> HRFRVCALGAAFCVARRWRSGGGPGDRRVRTDWYRCYPSLMEEKDRDMYHCYYPYLFDHGDKMSLYPKIPDNPREWQVEQLQTTYDAIREDKYDAFVRLRAKFPELYQDTYAWDNPPPFGEFNMFYSVRFGMIGVKAFTCKDYDDLGNQFDCTAFWFPDNQIVKHSTRNGDVGTDKVYVGAMNVPVEFHKPHVAAFYKAAGVPVKHVSAGFPVTPDAYAPVGTKLDVRHFKPGQEVTITFQNTDYGYQGVMFRHGFDGGYVWLGDSKWQRRPGCMGAEGQKRIYPGHRMAGQTGASAETYDGVPVWRIDYKNSLIYLPTLIDADVGTYVKFRDTINTKGYTLWNEHRGTPPFPTFIPSEEEDLSKLATDEGQLTSPPLYMYFRDEFAAAQLVTQADVEDAKSAKPATAAPKKKVYDLKKYTEARKKYRKNLQKARKYKLMGVRTRAHEKQQEARRAKILKYKRVKT;> MLRLTQAVLRVQSHQKKRAQHPNAGTRFGRVYNRGFVRYGFGGFGMSVYSSKKDRTFKVMPVPPPPPATTAVEQRDDFADNRGLSATTRTLSPTFRMFALEDGGVLVSHPSHAQIMRWNQRVHTEEGKAANSTVMDEYVNSRIQAIIADNTIENTSLSQWRKAHMWNVIKSHGKLQRRWGTPDFVMGARSTLYNN;> MSRNGELCLQRIIVSYSPNKGNPAMRQFMATHLPEFHRQYPQVKIDIRPRQWPESSITGIYRDGSEKAYSIRFLSSMGINVRFHRLVNEGNDYNHSFSASHLHLQRRSVQGTWNPYLWNYEGTRARHKPPAQWSRKLTEKEWDYYVQQYGAQMKAEEDTIADRVRRYTDIPEASTEEVNQRWKEHVMPRLQTDLEYNLSHWKKQHRTGAGRPAPPTLNEYSLFSVPDHSSLGQDAIDMLRRREAQREEDWWRERKGQLKPPE;> MRYCRPSRPLVLARASSVLSSSRTFHSQHRTPIIPQVHVHDEPTAQRIHVGYYLHRHPVVKHSPHPLETEMGYLLEREQQRYSRHESAESATAFFASRGQTIDILGRTDPNQIKGNFFGLELYQDAMKVVMQRYTPEKRLTSADLWQPNALGDAPPPRHTLHRKLDDFLYLIVQEGATGKWTIPHTARKDDESLRMTADRAISSQNSEGLDCYVWSNAPQATVFLKDDNTRLFIYAATYLAGRPQFASFEPKPKDHAWVTRHELLQYSDTFKSAELLKALLDISADGTFEA;> MQPRRMAGHFNPTPQANSLAATHYAHTPELRHMADGAAMSLSGQRIPLLKPTLSKWSRQLRSDIYDELLKLPLRYALHDFRTLQAHIHAVPATATNASCTAAAGERLPPGVYHASSGLSSASPDAPAYYAVAGRDSAVGYAPPLGPADPVDVIPFFVHRSSNGHLPGKVYSMNAKTLMPAFYMRIQNIEGDMFRFEEELMKIFPTKKIFVRSHSVYVYNVNLDGRAVLHHWLLGLGF;> MTAPASHYTFANLKKLGLCAPQVALSRQPRLRPHVGHLNGLVYPLPYYAMWRGNHDKYTYNQATPARWGEGNTNTMYHQHYAHAKCPTDYGRGGREFQFLSVKRGKLKRKPLPTVQYVDPNSKPQWVFKSWHNPLSAPSMWEREVQYPEHTPAHTGAKRPLAVVAPKTSHKHLFLMHMEKVTVTVSPLLFGYGHTLQKAALDFYRRGLSARSPFPSDKMFLYYSIDHITPKIEVTWLDGSVYVPPLIEGVKAQDLIQMVMEQAWLAADRMSAEGRVLNPIAIDDYKWEQLIAFKQKRAKGAEAAKGGAKKK;> MLRRSPVPRRYRTAWRELLHPLPVWARRQQWLKRDTVEMNEAILREPYYRIKTFAQPAAFVSPRVSESAAHEPDTQQSSRYGVDRQLRGPRRAVSPERLQELREQLQFVGSIGPKVPPAAGAGTAYQDEYGTRLRPRYPQSWDTVPPHQPSRSEI;> MAFRGSSARLAATPGVGIAPETTPVKYVPEMLNIQNAKWWNGRGKPVYRSTYNEKSWLEKARWGAFTKGSRPVMRQRYSAAALKEALEMVPEGFETCDVPRPPQRIRAQSEGVVGRWYTNYWTLHSVRYQCQLAGVEWQFGERQRPRTNYDEPHMYTDFEETKAIRDYRSRWINVNRSLVGMSRRMKESEEEARYLHFKKVQDTFWSNRKVLVNRIKSMHNQGTLQSAKDLPIKTINIKAFLAE;> MHLHISSIPHRNSNNSKGGVLDATGPMLSAKRGALLLQAYHRPGEVISYKAGDYHLVPKKFTVGKRIAVRSYLDRNRTELSDRTFMPQKNWFRPYDLQDGCFDRDHERLSYRFYNLETKVIWKAFDTPELIGMLLHDETVKGNSGMYAPDMLDAALHYTREARYWRCIGITKPFYDRNTLRAHCWEDNGLQVGTLVMSQAMRHALMDLERAVRRKELGLEPNYLWDRWGPIGFIDGARADYLPRFEHNPYVDPDGVDVTEIDVLPFNTHEQIRERYRDFIEPDTAPFEEVFRSPSHGSLTTLADIPNASVVALYKDLKLKAGTPVAGDAVELAPADVRTLFYLSANPEWRAVADGKASWEEVVDAMQPVQAELDEKIDAARLLQNTRHNAERVRAFFEEKCGFHDFMYTPDKTITAAVLCYLTELRRICTETAWGAALAKCLTDMERVQGMGRDAFLVYRHIEDAILDKKRRLWAGRFAGESHEESTLDYLLENFGRRAERPRNVGTTGVEFDREQEPIGRQVQRRVLDSDKANKLAEIRRSRGKMWSKKRSVFDALHEKQLQNFNYGVH;> MPAYSEVKGTCGTPVLDQLIGYYVNIQSRKMYYKDFLRIEHQAVRWAFADIRKNSEALAHGLLQTGVRPGDRVLAIQPCNCETFVLQLSCAKIGALLCIVPQDTISADKLRFYLNEFQPRHLVAREWINVPEMKQGELVERNMHFWDTIYNVIPELGLSYPGQKFQWVHSQEFYYLKKIIITDHNMNLLGVTPMRKMLVWGPFSYYEQRLRRLSALLHPDDPVLALEDPNPAMEDKLHITYSHRNCVNAGFLFGQLMQLKAETRFGVMPNHHTDPIGAIIAPYAALTSGAVLVHIHSDMFTDDHAINGIEKLCVEEVETLVGRKADFDLILKHAGNFDADQFEHLRSVVIFEDGIEAPVSEEYLNKLSKALSLDDVYVFRGPIEASYMLTWRTLKKGSQGMVPHVEAKVVGDRGTSDAKVLVAGTRGNLRLKGPHVTAGYYNNAGLMTELIDEHGFASTSREAMIDGKDNITLMSAQTY;> MCTRVFDVSQRFILLVSLPPLSLSLRPSCCSRKAATRRRRSTASVLLATDALSLFVRTHYPSPLLFLLLPNFPLPIHSPRKQMRAAVGAVLQPSSSVGALRCQARFITRLYTSYFKGELFPNQLARPLERLPRGVSLAAARKGQQAAAPSSSGSGNPATTASLDVVTWGDVDSTDLVHANEQSRAVAPQAGLAPRRPYVPLGEVAKLELQGDYLTEGGLHQEALEYYGVVAKAYELAYPKDHPQVAGIRLKLAGAFRRTGRLTSSKANCEAVLQMLDSAVQPPLELIVEALFELGLTSEAMSDAAAGTVFEEAVALVDMFHNSGQSHKMLRLLPRLGRRFNLNFEEKFVYFSPFDYDRVFALADQCLERAEVFYQARNDRAGVMRVLQQRKELIDKKFFNMRDFAGRIHTMRGHWKRRAQVLTNAPTPDELLRYSPTIHQVYRDFKYELNAPIGREKEVQPGVNRVVHDMGNPYRRSGVRSQRMFRDAEKNFEKYIRADAFEA;> MPTTVLYHGDQLGPRPLVILDHSVARLEQSATAVLDACQEAAKRYEAMLSSLAWDHGAVFVPLQVSIGEINVMEQSCRHVCAVLDAMDVQWSHVLAHSYGALVAARMAASTAYPHRIGSLLLLDTPLVTEQLVRNTKQREEIAKAKKDVNVPPAELSFAIESLRSALETTLPYPAAVDKSLYEDHLFSSASVFREKGLVRDEHRYVPVRHLAQVHHPLQLLVPVKQPITDVAIHREFFGLRRPAVIKTADNHEDLFSAKCADEVADVVRAWMQRFEPDVVMKRRFEKAAKEMVQLMGSSASFGEKGGGNIEKSEKKEKRKGRQ;> MLSSAHRAAFARPTATLWASARSFGAGPTRLLLGLEQVQDVPTSTDRKPTGMHRGPGKRQTAPKEAAQYQFIKKWDLQMRETWDELEPFKGLPKPKVQFGNEAAEVIWPYALLLENVIKVHPYTKSIYVYYSQRQSTPLGELAARVAKRVSQAYLIPITFHNSHVYVEAEMLLEYSETPWVVVHCLDGTHKLIPVKPQAGQTVKEGAEEVLNGIVSACNEIGSAVKNPKEVMRLLSERPLQNQYVRVNYQWYGDTPEERMSHLVKWDYEPEEVVPQLRNRTQHVLDWMNYDGNLPTHNSVRVNIHREAARMRKPNVSAGPKTFFNSSGSRANARTARFDNSRSSQS;> MLRRTEIALKKGWTHNPGHTRRGGKNLAWRPKISDAKLSQFVPLALVHPRRHPNNWQERQFNALGYTKWPKDIGFYNAGDNFEVTPEAAWRLYVHARDEPYWGKLHCEKTIITLLPVVEKAPKENMERVLDVFRHYLKRYGADHYIYNAVMQAAAFAKNYEQAEQLFKEMETLGLEPNAQSYVNMMLAAKLCGLPPEKSEAYFKRAVKDGAMQSVMRMDTEFRMWMDQLDRLGSFTASSGYLSVNEEGAKPMPRDMWAIWGWHRSESKFISRRDLIMQQVRARVHSGKELVGTVYTKTRRQPWAKFNGMLRHDYNGPSYRAPTIFPDAPEYTNEAGHKAF;> MLQCTALVLKSQHKNVLRKGRPHMQKYKELNRWQREAQGITKWEQGHSHRPQPYVERFNPEGAGLTRGTSAYAWKWWHTQYPWLPNVAPADYVPPSPRGIRPAAWDDEFADVVLSMSDEEIQSYLLDKLTEVIFAETQRDGYELRRLDFEGKPLTELPERRIIENFVFEEETLRERVLDRVVEGVFRLVPTSTDRLELKSVANIIDFVLTHVTVARKPLQHEIPEAARTVMRSHPLQPQLGFVHALPTDNRDAVVQEWERMHHLDWQFGKAVYEPRSAENERGNLTWLREVRHHEAREAFQADVDSGEARRRHMAKIKAAAQVPHTGTTSQ;> MLRTTHVSWASTAKGYMNRVMVYAHRRRKARYLAPKNAHVRSPLAHKMPEEYGNTWDPRSGVEWHNRMRNRNHYRHWPWARWTDDPVRFHQDSVCHRTVSALSTVANNGAPEWDYYAEVGQAYETPSHFPLSYTAPFIYQYTAQCWSREDLQSYLERIEQSSGLRTIADAASRREALYTWWHNAGMNVIPLGVLQHLELVSRDIVAQNARKSYRIEQHERGILRTPEMERYYALPHLRGPSMPVQLAQPSGKYPSGKFTQMMEDVAIHPLQKPDARYKHNMYPA;> MQRCLARLFQAGVHTPHGSRYNAARMKNWPVQEVPQNFNFTNEQRFKAKAVPRDTGKIPRDFLLSVLYRNQPCEVASLWEHCLHDPQIVLDSKRHLREVLQQARAEGFVSFEKDAVTDRWVCHLTRERFEEVRALVGARAEAQDLYSGLRGASATETSAYSESFREMNEDTKREHFRLLSEQVADTTTHLRKFQRMEMDYLPYTDLNGKVNFMWWYEMSDTRDATALPEAAAEGSPKLSE;> MLYGGSRVQYLVQPPFTLHKIRSENLPPPSLYAERHDLGLEMQLPRDMHVYNSINMAIQRQVGGDSSTLDGEQQQLQGGHADGFDMGAFFTEQHHPERHHNSSLPYAKHDTNNVLAMRLFPVNVGVRARTEAIRIRTDDCLQRLRDADLCAKMRLPLEHPLPLSRRSQYAAIHRVRQERCYDAPTEAAGERAAAAAEEASRTAHLRGAAAHPPPSELSIVTRPVDRLGSHSGSSAAACTADADHLSFPVHPFAAAAVSSGCHSARSGSAARLASQRWLPLQTLKPMGHNWSAATRSSGVRGPHMQLMQERLDQKGFGWKRKSRSLWQQDVATAGFRPHRYF;> MLRWSRLLREMAPELQLEYIPIIFTRTILGPQGGFAGEERLIKREVAQKYMSEGNAVTPSAEFHQGVWCYNPDSEQYDRFVERNAEFLDFAARKRQWLDVYWRVNTGYLLFGRQSWGQGWLLNCPLRKKDIAQKLWEQYKVRVDPRLIEFREKDRRTGIQDLGHNWCWLYLPGAEELAIDREVYDNKRVKVRMHIRKMSSYGALY;> MRRLPLFCRRPSRCCGATASGSGSSSAAVLAASAAPSVLVLAARGIATSGRVTNEDRRWWLVHLECAPDVTPGTFVSWLDCCGTHTTKKLIERNIWTIEQVAELDSDRVDELKYKEGCLKMDVVWEHARTIITPLKQREVSGGVESQLQSRILELRKKRELERQRELLARERATVSDKREETLRRLRESVAAKKAALRKKLDEQHGEATPAASESASTEAHRGTAEAAVEDEAVGNIVDRMSGGNPPRA;> MRPSALCLGGFTMKYKRGTGLWDEDHVNDFDANKYLSARSTMRWYYGMERLQTRNNMNARRATQSYNNNMGLHHSGRGAFERELERRGIQVDKYPLTTTTGAARVAEMVLLRRQELEAHAKKAMESQRQARRRDAPSEWYDETEGPLNPRFLASMQSNYTQVITELPSSPVTGRRELPGASFA;> MMLQHTSLLCRKALQSYPVPPRARNYERRWSSSRTNPYNRMFWRTVLNEDFARPSFWVSDFRHKYLAKHGMDYQGRVPASPAPGMYQGFSDVHKILANHPKPQRESRHLPVMPMTPRVVFEHAQEKRIDYAKKMHRDRRLVEQLRTHEFWGWYMKLQRVRGRWCKEHGVSSRGVYGPAVDAAELWG;> MFQRTCTPRLLACTSALLKRSGKPSDLPDYKQVYLPYDTAPTKTELDRERRKFMHAYSGRMEHRKMVEVKDVPQNMYTYGKEGMSIPISIFKDQADPVIGPEWTYPGIFENKIVAQHWYMEELFDREKSNTFESPWQRQVLDNQVKRRLGKVAWRMSMLNIKTIDIFHKERGASKRPGAGDTKAPATPAGKK;> MSSGAVGRGSFHSVVAGANPRRIPTYYNSAYELIQLHRAHREVTRNFLVRDKVFDNKFPGCSLANGLFKMVPNKRGNFHTRELTESIRHRTIWGQRIQQQRTINAAILEDATKVLSPAQMEDRFSYRTPDAAAYFSPQEYTAANNWPNYWQHPTEKHVVPKPRWRREPELGGITRVRDAVATPIADY;> MYFYRRIPSLASKMNHMRQFSLPRSSAAIIMAASTAALAVPCRAMHGKPASGHKVRTQHSRRWWMQSKAHHLTAVPHEEARSRPHFPAYTEDVDQPMVVPDGVCCFNCDKPIDGDDINSYVWVPSGNARVPTTQGYFFHVKCFKCWNCKYRIIHNQFYSKDSRAWCLSCALGRDIRVPTRRWHTSYVNTHRTGSRLTGQFFPRHRHQMEFLFSPKE;> MLRIGRTLLAEVTTINSTTASVSGRLIRIRKKSKWIDRRSTRVPHNGKDIWYFGDQPSCALCHIRFRYKQDYEAHKESELHVNRLRWVETMNWWRETGEPAYLKASNEQWEWFEQHVLPTKAQEMGCTLDEARRVYRQAIMTETPTWHRPLQCPTVKQEVQEPRDQRWPASPKW;> MLRFTQVIRKNPVVFKQGQGMFSHQLKRILNKKSLHKYNWDPLHMYDPRKLVHANRYVDHDTYEEKYDPHWEHNAHLVPDQQFYNIPVPKEYKDAYWWRDLQARRVQCPTEWVHFRMHTKDKLKYDFQDLAFRKKFEYSYEDVVANAKDMCS;> YDSRSSGVHDVAPRDGVDFMYEGPQQVLPGAHPLPLFHPDNSVTRPPVSPYLPSPQRPHPYFTTELPELPHFQTTRPIVYTVGTMKQRIVAPVFDLANNVTHTRELDPFIFGFYPETEEMAKNLSYWLVRCQNFSSKWDYENREIWRKAKKNWPNTGMGMARVGDRKNHAHPWGAHSKPVKPWNLLMPTMDVKTWSKSNRMLVTLKMLQGKLQIVERLTLPEPTQEAYLQLCRTMGWDVRHKGGGALFMDGGSRLTPSSEYDRAFFFGSFFNGRNKLVRPTLLCDEPYDYNRTSSKARTKGPKGQKNPIPINRFNAYDALTHDTLIITEGALLQLEDEMYTHKLAMLPPHIRAQLPERGFLDSEVLGDVPPALQTVQMEAAARTEEAEQAMYAPYYDNPYHPWQDEGEASYAVDAVEGTVQRYIKSRKTSWAMLS;> MAQWIPKTAWKVSNLNKRYGAPYVAKGYASLDPRCSLDAYSSFQQTVTSADMKKALLSIDSTSSGALVIDVRSEPERRLRPLLSPAIVALHPHDILSGAACPILPSNKERAEMFVVASEAQRAVNACTALRRWGFSRVTAVSVDAVSEAIAAVQKPADAATSSSTKS;> MLHRSCVLVDSFKEHYHRVHLPRRLALQRYIKREEARLSRHKGKAVAAAAAAGVQPGEVAYKYNRWWVSNDHEFVHQFAFVEDPDVTREKRNTLPLVTKENIWKEPQQTFFLPFAPFVRVVDYAKDPDTKFLKPVNIPRWKDYMQRTKPIVPRTWY;> MNDIYARRLAQTSMFHQLMRSHGTLWAATQVTKEKLNLAFVKEEMMRVNGRRAMPLLIGAAANENLNDTHFTHLTEHCAWTESARAFAVQRQTPLTQHIASMGRMAETITQAKTASTSQLLFNEHLARIDGISEFEEEPFVDDEDDS;> MSNRFFQKFYLRCGNCSAIQRSAQGYQPIANPILFKSDEHCRNYHDEQRRAAGYSGMVVTCRCHRCERVHSNWKVLDAQQFLDAKLRMTPEERAQRLWVSKS;> MLGGLRPLAAATRRTVGGALVSPALITPSRALSVRTEDFFSKEAVSHARRVSWAPHTTEKKVGAFAKLSRSNFNDPLPVSFQSEPYFEEEIEAYRAHHRPDVYVYKYNVSPTHLSLRE;> MRRTVRALYNSFERGWKDKTVHPLDRRGRFNLDEAAAELQLDEAYVASLYKPLHYTYSMKGQRYPAEQGRTSRPGSLAASRDRMFPLYRRNYKLNRELRVLDHRRISTD;> MLARYLDPSVHPLRVGQVVAYDYLHAAKTWQWTL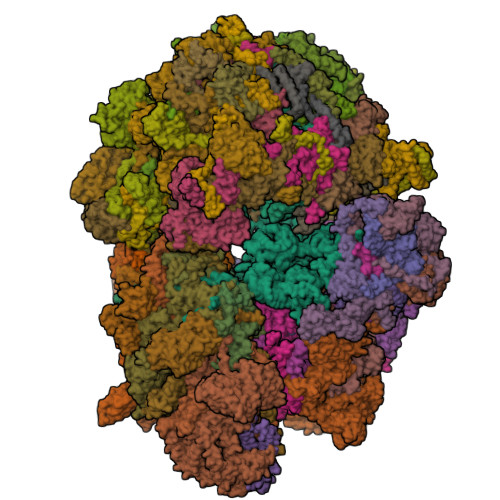GTVREIKDYTAVVQQWGLHTGDIDTLRSILLKEVDTENGRMKNYHDMLAIAREKLASIRRSNEDRVSHVRGHFDKAREKVELIDEVDLRKVTAQAAPSPVAVAVLKAVWAVAKCDPTAVEFYEWADVQLEYRKPAALDEIAKTDVLAKLYPSAESLQQSLEQDPKLNYKAAARDSPVVASLHAWVITALAYQQAYNLLAHDKRIQEQNDAIAAAIAGMKACRAKIAKLKDELSSKDTAALPGQVTSFTRTSVLVTIPLSAVISPVNVDTDVKRCVLTKDEVEQIPIDAKITRYAQKQKLAITGSHLLDQYAAATTTHIYVTELEDRLFFFQHYMASALRDAQTAAVDAHQRLAVSLHELEAFRQKRHDAKKARAAEPELADADGVEPSSGPTSSRSPTGRAAPRGQSAAPRGTASQQHKLLGPAYQSIDPATIANEPLYAVTIEEYKAKDAAGERAMDEAERMADEVQRLAVELEDAKAAADKLAEELAAKDEELAAHRQKRHDAQQARASDPALAAADAVAPRSGKGAASPHVGAVQRQAVDPATVPVAPAVIAEEPLYVATAEELQHVRDFADQLAEELEAFRQKRHDAKKARAAEPELADADGVEPSSGPTSSRSPTGRAAPRGQSAAPRGTASQQHKLLGPAYQSIDPATIANEPLYAVTIEEYKAKDAAGERAMDEAERMADEVQRLAVELEDAKAAADKLAEELAAKDEELAAHRQKRHDAQQARASDPALAAADAVAPRSGKGAASPHVGAVQRQAVDPATVPVAPAVIAEEPLYVATAEELQHVRDFADQLAEELEAFRQKRHDAKKARAAEPELADADGVEPSSGPTSSRSPTGRAAPRGQSAAPRGTASQQHKLLGPAYQSIDPATIANEPLYAVTIEEYKAKDAAGERAMDEAERMADEVQRLAVELEDAKAAADKLAEELAAKDEELAAHRQKRHDAQQARASDPALAAADAVAPRSGKGAASPHVGAVQRQAVDPATVPVAPAVIAEEPLYVATAEELQHVRDFADQAAHDAATREAEVAGTVENLRNELDDVREMNAKLEDEVFALKEQLSDAEDAYKKLAGALVVAEDERQELCDDLEAALDELEQKKDEYDELLGNLEEVQGLLEAADVAGRTAVEALEQRNRDMADLQGELANALDASKENENLRALLDAKEREIDRLKEYNSFWTDTVGTGKQKVTHRLTKIFDGDWTRLMRHRPEALKAAFVIDSSNACHVPGDQIFLVSNSFTRRLLTRTDHCPKCDRLSTFRFMSVSGMVGRMPYKPVDTPGPSYATLYWRKQRSGKIASQPLNEVCNKNEF;> MWRLSRVALQSNRAALYMPYTPVATNPVVYFDITAEGDALGRVSVELFRDVVPRTSENFRSLCTGERGYGQCLLYYKGTPFHRIIPGFVMQGGDILTKDGRSNVSVFGYPFPDESFEGKAGKHLPGTVGMAHSGPNQNGSQFFFNLGRNEQLDRKFVVVGQVLGGWEIVNQVVKLCGSRCGTPVSRAWISDCGQSGGYMAEETQEALQGERAQHVIPGKEVLDLIQPRY;> MRVWVLAPHSLPPASFRPIFEARPPSSPTHSFHLLPTPIYLYITCTDAVDLYVCAVTSLLAEWTTTMFARSTIRWAAGAGHAFMDIAIGSQPPHRVTFELFTKRCPIASENFLKLCTGENVLPQVSSIDGIGEPSFRDQFLPQLTYRNTTVHRVCKGYLVQGGDIVSGQGTGQLSIYGESFDAPEEVKASKFDRMGLLGTAVSAPHLNGSQFFILTADKAPHLNGTCICFGRVVDGWTVVKAIEAIPLTAAGEPAERVVVVECGKL;> MASVSPLLMPCRGVKLVNPIGKQGSQHYGLEPKLEAGRDTQLKHTEMYDGYTDDFGVFKEGPPVTLRLEYVRSPDHGYSQHILQKDIWSPFQVGANMMSYTPLYYDWKGFSSRDYFGHRSGTNPGSKVLLGHYRRDEVRSWGYRIMVNHKPQKRIPKWLACVVHIPRKKTFLGFFLYANGAYVAELLTYKQLPRIIYNKAFQGCLPTIGQTVSLTEVTYGKEIHSVEMYPGHGGVICRASGTAAVVLRGSEPNLVPLLLPSKEVRLFDNMCHAVFGRRAGVMYNKQRNFSKRSVEENMPHRPKVHSKTKRVSSHPAGGGNGGSPNLLTPLDWRIHPRNCVKTKYWLSGYILRGRQYNRNQTVADLKSKTYSWANRDPVYR;> MSVFPGLCGDVATTNYRVFLGTLPNLAVEERFLRQVQPVFPWYASRKHVKEQASEFLEIDLASCDPELLLRYTHVYYVRRQLYDELVDRQLTLMETGKAAKVADSALLTCLAQVNAAITPRLQYELHLLQQAKKACRVPRRRELNPDAALEAHDYLCMMRVVEEDVGGIPDAEMQARAYLPREVLEAKVKELAAMIFGDGGSATKGTGAALERKEQKLLQRMIPADYNKVGAVEKLRPVDVTALYRFTGERVCGRPADKPFARALWGHVFRKVGSHPLYLQRASLYWARHSGLDPQSATSAMPADLATAVCVQQALFPALKYRCQYLYTSPDIARQQWRTGHVVPLLRLFPLLGAPAAEDLAAQLVVEGEWAKLGIEADTNLLHDTVLRQLKDMVEQVSALYESDAGAVLKRVEDGAKVLCPSLSERESLTMRGAPEDTSREVSAAAAARVANAAPA;> MLRFFRARLAPTTTDAAAKLPAGNPVNKTWFRHNLIIRRKGSYRSRWGNGTEGYGAGVPLSDQVKLHCVDNTNCKHVRLIAKATAERFAHCRVFPAVAHRVSVQRFKGRGGGGEVSRHRVKPGNIYWVCLFTRRQTNTRMSGLQTNFDRNTCIIMNDQRVPLGTRVMYCAGRHVNHKYHLKAVVLANFFV;> MRRRDWCGVCLPAATLHALARRYSEYRSSYTGARSAPWAAPEAAPAYPSARSPFPLERPRFRKTHIEWMLHHGHGDRYGKYGPSREIADFEYADGTPSSISGKRFALKHHQDHLLVQLIRSAAIVERFEEEELLPRIPGTPEQRSWDPEIPLFLEDVDEFGRPPRPVAGNMVARVIEERFAQESGRTPVNLANKHAGEVLEPNTMFATYDPAAFVSDDIKKDVRRPFWSRRRWALSDNFMVPMSPKPKNTIKDE;> MVLNKWAAVTKSAPPAAGLRPLARTVSPNPKLRPADYKVPYVLRTFIKDRHSSEMQHIENRGMYREELAIERSRFPRMQKTLTIQTDGSLNEREFEFAVPPVVMLFQDRLSAHRQRQVALAKIGKLKRVKSWETSVRGKESLNPVCNALVFPYCVPKKMLVRPRIVDPLSAKSMADNRRSRDDPS;> RRSAWVFVAPWVPPPRHDVKVTMPPPPGGEVGGSYGVSTGYSDRLARTPYWKRMALSTYALRMKENETRYPMSPHREGEYDLRYTVTAYPDHIKHRPLLEIGEAHQIPTIEIPVIFLVNLWDEERLTWFGRQYETVYVNRNVAREELLPQRYAIYATEEAYKLLGLPVVNHSIHEEIPKTPHAYKKLLEKQSYTEERWKYTIEYLFRKYEADPPELQDKSEDGWDGVEELATSATAGGAGDSLAKRKGPVKQRKARKIKLF;> MFSRGAAATAMAKVSRLVSPRLRIIHRDYLTRRGGRTHQRCSAVAVDYTPTYFATYKSDPGQCPRLIDAEAVHGDEQAFWSARRDFYRGGASRSYYPAWDRQAQALIMLTREVPRIPQEAAFRLFTLGLKMMLLPRLVAGVELMLPSWVTMNAESVLNEGLEGKVAEADGDGKATGAAADAAALPSASSAGANEDSGSANAEKR;> LRRSAVRYLKARPKTVNIEPGSNRFLDPNVEAKAKDIFAVPEFPNKAVLHNWRFFIKAGKAATGPPVGQEFSKLGLKAMDFAKAFNDRTKPHFKDDIELIVRIQVYFDKSYIFRIEPPPTAWFLLRAIRKKRGETGPVVLRGNYCAYLTLEMCYEIAKMKQMSWGKVEYPPIEVRVRRVVGQARRMGIAIIGIDTVHSSPVKGMTEKQYLEESEKHRKVHMIQYEALKAKELESAPLIERLHRPNMAPLTNTQLEEGLKDANLLNALWKSSHPKSLFTQDTRDREMARRYLNTRGWFKEMTPEEMRVVFLNYRLPKQEDHQRQLNMTNGQAQSQAYWSRDAASPQ;> MSKQWLCREGERWWLLDARGQQLPHVAKIAAQYMTGQHRPDFTPGMMTGDHVVITNIKDAVMTGDNWIRVPITWQTAYPGGKYRVRLSEMYERDPCMVMWWYLKDEVNRHFVRKLKTRTAPLEKAWLYEDSVHPHAEKNPRPLVWTDTATMGWRYKDPTFQRRWSPNQFMS;> LSISAVQRRYRLFHPVHQTVPFHFNPVQSIFPLIYENNLLAKPRLSWKDYEGRKEFDADHPLPVVGTRLNERTTTHKWSHWDQYINPQITQSWMYLTQTPEYVGPRSGHNVIKMGWMKIGGSWKYSRSYNDARRGFAKGQWQERKMTPRFMLAPRVSAGGPRNRYEGKASFSRLSLSKLLWAVDTGRLNPNETITLYHLRNAKVIADREVVWPGMVLLAGNVERVPYPLHIELQNASAKAIQLLEEAGGSFTNVYMSHEGLYQELHPEEFPTFMEQELPERKGLENFATNSRKRGWLAQWYEDESRYAHPGAGRRTAHYIRPPTDRDFPATIEEYELAKHHQKWHLNQPGSATVLPWHSLNTADMARRSAGRL;> QSSALRPSSLLRAYHYVHPKTGRPIRQYRKYGDPRFINNEVALIKGLFALITTDFGMVTQSQLENARLAILRRMPRGSFALTMHTDYEEFPVVQKSPESRMGAGKSNIHHFAYKFTTGVPLFEITALSSRRLNQAEAEGIFLAGRSFIPLQTAVVPRGRVDEYHVFK;> LRWSRLLRGRPPPVMGHAKRMRFAGVDDNPSVTHKPWDTSEPLMADYGWERGKLPKFRARSPFHRQQIARRMVTELIRKDYVIVGGARAPALRILADHVVELAKAGDTDSRQQLAYFLHDPLMVDKAFDEYPRRFRDMNAKYAMMTRLKGRRRSDNVAMYFVEYKNRDMSDNHKGEDYTAGPERFFLPPRIIETEKGIQRPPHMQMAFDRWASKFKTEEFHHWWRLRHAKLRYWGVRNVPHPSDVDPLWTEKEEEEWHNEMLANTSDFEDFDLDDDSYEAAGEGGSQGGSSSLSGIGPEPQKKY;> GYTRERTNRHFFVSRANAFFSRLPISRIQRALAMEAIKKGSMKPWKHTKEQIIGSPITCNFEYNPRPVRLIGTVMDAHTEETSIKGGLKVYARSEEANMMLWIPAGNPKLKYEVTAAKGSFEHYLDERSKWDEAWLTGRARMK;> LRSTGVSLYYRATAELDRLRGMLRGRARLERKVGLKRITFLMRTQTRYRVEQKAHWERAIVRKNVDSAAHEHGSGWQHLRNDLARQNLMLLPRTQQQLAQYEPLAFRAVMELCASRVAPPPPPMTAQVPEEAYATRPEDPKVAHPAARRQLEECVERMLCTGRSDVLQREGPRTTQAWMDAWKEYDLGSAAQK;> LRSANPTIAKALQPLIEGPKFAVVYCGNHQYKVSPGDVIAVQRLRAPIGSQIALKKVLMVGGPRFTAIGRPLLEHVRVTADVEEQKRMRNVVSLFSTPGRRRLRWLDAQHAATILRIREVVYEPTVVGELDKYDGVLLKDFHADRHPNPVFTANDGYDLYYPKDWNKVEEASAFLEMMEAPPTEK;> PKPAPRYNIGLRPAPKRQNVGGQFLATQKHYARELWYKRQYYSTRPFAIQKHMGSTPRILLDRTLWRSCWLTKSNLPDVNRWEKVVNSQRVTEDRWALVEEDGVMYQVNWKMYCERLETELQKAQDQLPQYSFMMKAVPSAWKKLDIELSVLRGLSVREAMAQCKLSPRKGHMAVFRALEVAQQGAEGKGLDKEHLRIAYITCMPGPTDKQVDIRSRGYYAWKTKKSSHLLLTLAEDPEMVLPDRTAIPYASLMTMKRAGLRTEPTMLDVPAITAEGI;> KRLSSHHAIVCGAASATAASTRFGDVVGGGSSCTATSPLFAAQRGRFYRPLVNQGINLWRSRMGRLHKGWTTWEYNRDVIPDPRPFPEPAVNNYFGRSRIWNPIAGKIGLVNRKAEEWGWPHQRPPPTGLRRSPEYFPFFFSRYFPDVEVRLVLDSVLNNETTRPIFHIPQDMSKQELVNYLKNIYNIDNVVRIRVRNMRGRRFKNEVGEIKSLPDYKVAVVELDSPVSIVFKQIKGTEDTPDNKPAAQIT;> GCVRVRTGCRIRCVRASFTYTQAQMYARYRTRSRFYKRPEKMLKAYNVSPNLLRLPKVKPGLLKGIYTDEKIDLRDRERLELVESIRHPKERDFYQDHTYHNQWIARDLESHQKIQIAGRYPYFSPDYEIKPWIWYPGDTVEVVSGEGAGQRGAIIAVVKYKNEILVQNVNVQDVVIPASETRPEQVVQREHPISVLRVRHVDPSTNQLCHLEIVKVRNKETGELEERRISLESGALLPIPAPEETVEAGDPLKDTAIQDADEETYDREKEMPLLVVRRLQAMENYFVDSLQKSHEYHKALQMRNAQDMQTFQKDVLVRATEKLAAAAAVAGHGAMAEAGSQAASVATESSQAGDAEEDAVKGTITVETVVAEVLKSEQRFRSDAAAPGVPGWWQNMIDAYVSVLEEEEATIEAEAAAQAQAAEADRRAEQLMADATAEAGQSMEEDGTMEGGDEDLDEQDGDLDEDASRSDRSK;> LRITPSRYASKVTAGNAKNQAGSPRQKAKLFHVIPGTPVTPVEKLKEQRRRFGQDRYSRQPEYRPGRNVRMDPNTFTLYATTKGVMTIRTSRINPSYKWLDVEPDIQKVYRSRCMRAALQARGKASMMVAGNVHYRAELDHVTEPHWRERVMRVPKATERFQDPNYFTRGLVPSLRPLSRYSYE;> LRQSSLLCFSTFALNPETSRAPHGPPRGLINRYISMGLPPWAAWCNRVNRHALYRMSDVSPRSFLPKAPHEMDVIWMNERVRERVRTSRQVQHVYRQLKYPFVKTGIHYSDTLDHWVQVPMVEAAMFEIEKDGGFDNFILKRSGPELRSTYGERIRRHLLVRQKETQKNFVLDQQAKALAEVTQAELMKATSEEELDAVLAKYGMDAEEFKRLMAKRVMEQRKSVAAAGLRSK;> RCSARRANVAALYEFVDGNFLNNKRPAIPGGAWPLESLRRKSLADLQQIWLSLLKERNMLSTIKEHYLRHQEELGAMPAPSRLKMVEESMENVKRVVKERDAEATAEAVRIFKERLAKGIYRYPPGPPPPPGAHDPTSTVKLVLSRRVDEERLRELLGRFNVFEAHKGIVKLTMQLPEDVLTQKRDAEQLWQQYMAERRNVEEYYKWPGSSTGSAESASVYDHTVVELAPGVYSGHRGTSAIESNCVDDSNDGAHGVVQAARLPVPPPKTRPPPPRNPLEHIKYQQRSVLSKAVIQLGYFPNITTTAPRFTKADDVPRPVHPDEIEGPWEVRVTYDAKDGLAYVQSLSLTSIDGAAVLSVEEEFPAAAQPYAAVDPVYQEAVRREMAQEETLMKWPNVPKWKYQYDLYTKKHLAQVVQYNYSNVVDYVDREVLLTGRSVWESPIDIDPTCGGMKSVPAHAKKPKRYMTHGLAEVGVTDI;> RRCVMAKGEDPAHVAGWDDRQDAVEWWWTEANDSRGRQRLEAAAAVAAAAASSTVGLPLFPRFSPGRRRRRRPPAPPPPPPPLFLSRHLHSMPWLWCTCVKMQMYYTPTALTCPLSNSLAAHVGHIIVGVAALLPYSMLLFLTVMCNPRKHEPVLRAQRIRWLTFHSLMFRLLRCITASPAVAASVAVAAAQTPTSLRPAAVCRRGVHLAPSVLAASAPPPPPQQQQQPTSAAVPASTATSTTTIAAGPYRRVGNVFIVTCIDHPFKFSWEVNRMLRELRLEFMGQTTVVPDIPPVRKRIWRVRHVVRVDQLDLDEAKALIGIPEHISFRDLAGQIPPTFGRGGSVANPHMRSKMNFMRLRRMRLRDVMHRDQLEKRLLEERHHALQQQQQQQQGGGEAAAAAAATTA;> LQRTTLRCYSALVGQATPVLLGSKGGTPKRKKNPMQLRRKTYGLHFKERYLKLEEWYFCPLCAEPKKQGEWCRREDCRQIKP;> FRASCTLLGHGQYKTRLKKRMVGFIPKVIPRKIRNNMVALRSEANTGHMEGYIKTEAERLDATGRKLQKTMWDPVLQRYTLMKETKVRGPFLTKSNIARKVDFPVGALHGTKLGGKK;> FRISLICFPKAGCEEITRQGRRVVLKPQEYFAQHRMQVWQMRFKEMGPPFSRVWVALGGKMRRRRIGRQIDVKDMRYYWRPIEPQYQRLYMSRLRIKDHSNKRVQPMRLRATNNDIGQASSLKEWERSSDRKYGAALAPPKKRDFEFRVF;> LQYTSSARQALRATALVLNFFPLGYTCGPKNKQVFFPPNNLDGRTTHQMKKLQGSTDKHPGLVPRDKLKLHCEFCRFHWVQDTLVVRCAAHPKEHNQREIWLEPTWTWGKQQPYQYYKYMPVNINPRTGMPLAREDAKGMNNERRSQGLPTKTRLLERERRGISRAITGLGIYNQRWQTRFPFAT;> RRFLPSSVAAWGAGRVLQCAAEWYHMPGWKTQSSTKDARSREQRERDRKARQIEKLPRPEALHDFQYPYEKTILSDSMFEYPVYETELDTPQLFNLTPPPDFFIYWNATDFDRTAYPPVPEDDHRVLVPSSQSPRWIEHRARLLQYLRKHEIMPHYVPHIHANVNLSVVFPGQYNTRARLTDENGDKIPPPPAQTKMTPRNFWFTAHCGNYMELTDVQQPPSVFFFEEAPAAASAASDAGEAGDAANKQSSHAAVNYYTFVMLSPDYPYRVPLLQDRHKADRGFFLNYMVANLRAPQAVSTVDGAVVDTEGLQSKGDVVVPYVAPLPTEDAGTTRHLCLLFKQTGHVPSVKPMTATEEQRDFPLAQRSNYRLHSALTKQTGLKMPPSASTACLASLRSVERAIPADPCAVSFFTTKWDIQVQEYYEKVGLPEPAAPVDEEIEALLEFHAMRPEKLRVRARHRPDGSVNMGDDPNFWAQALPTRAMDGSMQRGLGWSRRTTMGANGVPVVYPH;> MWTLSRPCLAAVRTAVLCQKKQTAAGYMASAGKVGNEEKWAQAAMEYIHEKNHVNDARKRQQDVDQERSIANAYDRYSAVSEAKFDERLSRLIARMSEALEEMRNLGLEEALEEAVLLNSEQPPGHYRRPSLTPPLAGYEPGFGLDVPQLRSQQAEYPPLRRPTDWLEFGEGGADDFPYVDTHKIEDLTAKHEAQLEEQHGVLREAAPLTGVEGEGWEAYVALHRKALARQHLIMDLHNDPELRDKYNADEAFRAAEWERRGMGALSIEAPLERDLELHYAQVPAYEAFRSH;> MLWCTGPRRIVFHNAPSVYPFTKPFHDTPYDQDRGRFDKTKNILRENKWPAWMDHGADGTGFGIGLNRTHPLSKLRGNLRRNPSEIPRVLNMMIQGVWHKSGNKLYFRGGKPPNPSTHPYLTGEPCPVYGWKVTDPGVIREFNLPQPEDKTRYKPYVALQERKIMGMQAPTKEHSAASTSAASTDSKPLMKRLFFWK;> MLRPTCPVAKNLTSFATKGTMRGGIPRIYYTWMKPGSATRRRFEKMRNPFVNLETGTSLYFRDTRDSAEAVAHAADSKGLKGMDNGVDLYNEYKIVPDLYPEGFQWKHKLNTEYNQWRSNTWLTPELIPQEHRGRFLCNFQLNIVAYDMRVVKFSPKDHRQWIYCVLYVGTGKGIAGFGRAVAPSTQEARNEAIREAFSNIIAVDLEQEGPMYPVRINADGARVLLYPARRIIANFRVADILCAFGFQNAGCKINLKASNNPKAPTHTVEGVFEAVKALRSVSEIAASRGKVPHSLVYNIYPYLEEMRRRKGMMAMHPPGKDGIFMPNRVVDNRMPDHLKKGYYDDVYWKDFFAGSKEQLNEPKMGLRGDELRAQLEESQGRTAKRSNRRTLDDVLRRLGKTSRDLGALQVVNPRLDAKLPTHMKRNYLLH;> MLRARARSAYTVARSSAARCSAAASIGAGSGALNGSTGLGSGVGAGAASASLHEPRRYSFKYATKRQHNEARQPSYIHDKRYGLFSNEHNIGKSRRGLPHITPIYTKHMSLWETDTDASTNRFFRHYVFGQREEHLLLGRPHGFEADQAGGRQGDSAYELNTDQRYKGVPRPAITNLHYEPVWNQTLYRNTAHGNQLTNPSSKLTAAVLGPDLMEVRDIKSVEHCKAWFDRLSFLIQQHYDAVGDIGAFRSRHAQHVHEFFVAFHDALSSFDFQDRYLYDQFAKARPKHLEDLFAIFLEMEANYVNEAYCPRCSLPYATTRYCGEGDPNTPFRKHRGRWAPHQYWGKEWYDVVMRRAEALWYRATEDPFFGTTAHTQRQAEALLSVYVKTKHRAKMVDFLHALRGSKEFLLGQLQITPAMQKAADDLLDSTPHEHLLTNAFKLESSAAKYTGDAQSVPHSPLQMRLDMEMNKYRRQQREEGVVRVPPASWKLDTSAIVPYKVDPQTKHVANWRAVKEGIEQSFLATGLPKEAYTSEEWREMLYLKERIASRGARRAQLEAERQAEEAAMAKKYGQRSPAATSSSSWCVFPDTAWYRVFETAAEALKPYGVTHAGQRVLMRSQTYANPAAVPYTDPVRNASVLLDTTPEACSVFGGFESGEVLRLTPKEPEGAAAFDVVVVGVDKSGAEAEWSLYAMHRDVASQTSKGLLNLGTDCLQLLSSYAKVETTRRRAVLTVLDAQRTLPEEHLGQVVGVRRGELYVQWHLQRGGSSELDRSVAVPLGNPETVKQLYKLQTLTDADGAPALLQEPPSWRTPFRNDFVDERLKELEQAPFKREQWASLIQGKYTPKVKKYGYAQHTTQDDFQTKEYKDRLLARQYFHSPQAFSVIPERHERSVKFMGKWEHQRVCGLPTADRDELEKGWGEAEEISDAAVGAIEQALRDISGRRPGNFVKSPTETQSLRLNESWWTPLEFGWEEHNREQMAFLDSSERSIVEGARLPFGGKRPPFGTTYGMGERISEIAADYAKGFGLGPHGHSPQHDTAHFNTLEAEQQRVKVLGLGNALVRLFHEKLGNQDIQAWSLQQCGESDANVRQLLLSVEEWRTKGRAPSLLLRKVLQRYLKEELDAFNSGLPAHVPRLAVPCADASAADSIGSSSAGCIWVDVDRNAFALEHASQFRRGDSDEPYIVGLVQRAGMSSGSGGALAASPAGSGADNTYAEYIQQDVLQRFEIGLARIVGRGIPSSIIMERTVKNSRGLERESAKMLTLVLVGELAKLLSKMRVTPDNISMVVRGLAQCPEKELLGGGDFAVPVSLIFSWNGPQSNVSAATSNSSSSNANAGASRGAGISAVQQMLERTRHGSSPGSSGSGDGEKMVGKVLEELAWSQDGVAADVLYALQQNKANPTLRQEFLNAFLPVCSNDHQKAQHMYADYTLGKFVPNITVAIEAFVKFLGNISTHPGQLTSDVEYFEVDNARRADGTEGTGQYTQVRLLPPEIGPFQYENTLIESIETAERFRRYGILAGPARVPASGFIAANCKSLTYMTHRDKEVVYVTTENDQGLANALRSSALFKSIASNPKLSYLLKGITGGAPSHPLLVDSFNRFFYRVAPMLSFYQSLLQEYSATMPSAQAEAQIANFGLARALESEASTAIEQDFRRNAERYWRNVLEGRSTEEAALSSGGRESASAQGRRPSQQGSGRAGQSGSGSRRGSGEFNLASVVGHRAAAGARSEKSRVPVSSSSSSSSSTVATAASTSTRVKGLLGSLKGGGSGAGRGKGSRPASPSGVASGSRGGRSSSSNNSGDKNGSTSGRK;> MSSAGSAAPPPPHTSSFGADVELPMSDWALRLQRELMSPVDPLGGLAHKDYYRDPATGYAPQYAPRDFVHGGSIAYPHMQGSGSAHDSYAAAAARRNWLEHDVESMAFMSQDARATARQLSSDAEREAFTQRHVPADRHRSAFPGNASLAAMDQLRTSGPQSDEKVYQQAILDRYRAAATSSSSSTAPGVSYTAATGLSGGELVDALAEDYAAAVDDGMDEELRIAHGLRAKERFDFKVMQRTSRVPFQGYDMDRFAAQREGRPHGAQQLPPVIPPSSMEEAMKNMRGGAAALLDTEAQAWQTYAQNTTSEEPKLGEALTGDVINSLHARRWSAQHAKEQARKQRFGLGRQGALVQDGGPDRRTLKKHTNDERLLDAVNFASDAYRRTITDEHVDPYVRRSTERGVGHLLTNSFDMARREDRVAHGQQDLTERNTVHYGVPIQQSIDEFVLSHRNARGERPLDYFKPFPDFRAQRLIRMYRDIEGFSLLKQRPEAFEWELFTRYRAHHQQRRELALLHGLEPVANETAAERTARRLALDELCEKTPFDPSKLHLNDDEVEIDAETLRNWFGVYVLPSPTIVESVVRAEGGALNLHLQHAADEMNTADTREHILSSRYMNRLLLFEGFQHRWNRGFTKEVAGKAPEPVIKYAQPQEVLKYFDSDERAMYQQYVQQESDAQLSEWAKVTRGRRYIAEKEQYGEVAGQGYKVPVVDVQHQETGAVLTVSSKLVEKSAAAALADKKLAGGSSSSTTSSSSMVHFDGQAYFVLPGSKRTVTPLSIRLESGESMEMTDEVFSAYPLEVSASAKYNHALNYGIGEYDYNRGNYIETQDAIWEKATADQEEGWSPATHADGLCPGLPVRARRRLAAAGEDKTGAAITGDFQRGRIVQYYRQPFFNPDPRLVTVAFYADGVVQEVPLANVMIWQRRYHGPERTVGDESRRYNPAGLRRYIDVADPNNKKLSPSSSAGAGANGAGDHFLEKYEGRLTNSVAASRYRTTKQITEIDQWNRFDTSRADNHRPLSISHRRDYVRQGYLPRYTPWEWIAIQEADQPIIHETMRTDNIGASYFFSLNRSWRYKARPHGYLRNYENEVRDMLQFVDGVTPWKQAQKIRTYWEVRQHHPMPQFNRPEVAMHRNSAGLLPSHMWEMDKKTGKVRAVKDSVRDYQTKIPVPKWVQL;> MQCHHNVLVGWANSGSSTAAFLTQQQQQPLPPSPLRFLWADQPLGSPSVLAPGCGMYRARSCGVVAASAAAPRVRTALDMVIRSYTPIYAPDPATDHLGALRSADECRTLWAQHIPVPSLTRAIELWLRFGNDPVVHTAASTASAERAEGDAAPSSTSPFAYVEDYMGSNMVTGTPEHVKESAELWSEYFETKYVRRMRQSRRTSKQYVGVLGAAGRGRGAGESGGGSASSSIANLLLDEADHPNTKWEADTFFCEVAYLSERHLKTRVTNHLQLDKLLWGGTAKPDAFVQFFEAFQQQTITRIPLPVPSIWVHESTEAKKKWAEHYLPACSAAHEFFQEKLRPHAADAAAQAKLLADVAAAYRQVHAILLERRARQVQAGVYPSTWTGGGAAATATEEAWAANEAEKEQRRMDEGVYDPEDLLDTTAEWATEHAKIQAILEQPLTSSGSNGEKSYGFSLQDFWLHTERREALETVHVLESESLARVAAAARRRLYSETPLPDVFAGLEESVAKARLDLRAAVLKPHFNSVWCRMHYVKFGAASLVQHTHTASRQLLFHYAASTQVVAATAEMYYATKPLSSQLDYASPYTFRRSLARHCTRYGVEMAHAAQQPLLLSAAYLAKAEGVIGRVARQAAAPFGARRRARYSAAQLNNQRLLNPVKSVQVTAPAPELLAAGADLLTILREERTPKAKAAGEALKVWPLGSRQTVSYDWTSPALDKLRLTDSSLTAEQAAQRDQLRQAGRLEISLWRRRTAEERQKVRAEMKKEAVDVQALVAETPVLQEVLAYASHLYRKLTREQEQEQSYSDTVPTPHAWDEASGEWVFAVMLDDDVPLSETQSTEVFLPYVDAAGRRLPNGEYRVAVRAVDRELNPTEHPTLMSAATSSPFSVVDALPQLYAQYTRHPQPADKATGTPTEAPLEGDVAGKDLMSFCAFLREAGLHISLSAEFAMGQSLDKQGNVSVAEVAAVLRGTEYHRSQCEHGITDAQRTIEPQCRLHWSLYHPGATEQEWAAARRRVLRRAMAEERDWWLPDPMLEVTDVRTDSAGAASFSFGAYPAVARYGTELCTVLPAHGSNHMEYAVLPPPPGVKATARGIGAQVQAECTVDGTGAIASLHYGAPISAADVTVEDALRAAMEAIQVAQMRHNTLSMVKLCAFEKQAQTMLFCGIQGLEFGGKHGRTYAYALEKAKREMAATAEAGQVASLQAADAEKLRLSDQEQTSAAVDRFASQTNPEQRLTRFVPRSTMSGYSMEDVGPERASTWGL;> MMRHTVVRHHRTGKARAFIMRDPSLKILRAGSGFQQLKRMGMPSQKTLGYRQVDNFYANNQYQHAWPLLTHDDLGNSDQSNQTKNILYSMYMPKRNKGTAPWFRGADTYSVKYCEQGRYEYQRYLMINRFPSEYKRHFLRFLGNIRGSKSRDAVPQEALHWLLRMIVDNFNPQHVHYIAAMRTLQDSGELDMARDVWKIMERQQTWPDTATICAYLDVCVEAGEKTWAVEAWNRYCTELRFLQAGEVDPKPITRTPFSLTREELLYLPKWKKHFDHDPNLDVPDLNRFNRTREVYLRMAKVMLASDDMSMFEHFFDKLQAAMLTTPTPVPEPPNPHLVRRPRWSPYEHQKSLHHSPWRMDNNGRAMALGPSRTIEGEMQSRFFSNPQFLVHAVKEAVAVVLQRHMAMFPEATDAQTAAPAFFELTETAQETLAFCDGLVQRMMERLEDKLGSLGTSSLLSTLLCIRRVVGKQSGRALLEYANQFLAKKATLSADGLRESLTAPNYFQILAAYADESAYHYDPKTRQYTYAPGFRPTETMKGLSATLNEISANQHVAWSAEMHLQVVRTLVGCGTMKANAYFVENVLRQFKWDSRFLEALYAEYRRHNTVDGWAELTKRALVWTARYNVIASERLKRLIEDDYDIIHVQTRTFRELAVFQFRDAEEKRHARDVVNELPNPWIDYVTHALPFPDRDAGYPDEYGDIGQWRAPGGPGSPVKGPGYYAPPMEGEHMRGYTAEWRDLKNPMKPPAFPEPWERKYKQYARGQHPSYDMVYAGPMPEIFPGRRDFRKPTRWDYHDVEKQGKHKISGPY;> MSVIGVFSKGRATGHASVMSVLRYVPRARVPWQPSRFGRENLADDDMAQLWGTGRYRTGPGNYNSGYSTKKTHALEDSTVSIIPKHELEKFMPDISLGSKALVTPVSLMSARNGHRVTHDLIHSYDPYIGRLQKPAVVDHDNITVEDPNRVGLNAATLDCRSRIYRWLRRGPFFQEDNYFRRSTKLQRNGPVPVSVHEVPLMQRIIRLARRGHLKAACEEYRRVTSVPPVDVYRALTAACVPGAKLADAIAIFEDGHSRLFYVARDGEVLHNMLRCAIRAKHRVRVMWVYNVMVGRHYENVVVRAEVDVIWRYRIASLALEYLLDSNAGEEARTVYDYLVENELVDCDLHVRLGHVMQQALKEGKTVHVQQDALDGMALSQNVVAVAPQVAVAVYARYLETMQEGAAWTDARGLPLTDPAKTGADTNGAAAVAWLKAAFPDIDPVAVLRLARFRRSSKDLMAKDRPVYVQRAAQWVELLSSAHQTREEAPLTYLRKSRPSMANPNVRVAWLPERQRAHALLASDEGFKFAYAGPHTRFVEETFAYGENTLQSRYLAQQPVHTEVTPSVALGAAAVAAGMSSGSALPRLPGSSAAPQILHASVLLDGSLNGSSGSGTSTLRSGRNESAKAAASPTAGISSRPSSASSSAGLDDTHF;> MLFVLQCTAHTHTHTHTCRPQHLVAPLASLCRSLVVVSASLSPFHRPSLRVGHTVQCQARSHVSPLPTHLLFSSLALAACAHARRACRGAFSYLTATTITITVTTTFTTFFLFSVVLHPRFNGDRAAKAKTGKKMWRRSCCVLAPSIPRSVWDPAHYNENWVDSYSTSIADRRHWPAKKWSIGLEPRTPRDWLRFSYRNLAYAYNGALRACATFPEMLVYYKEMKQRGVKVDVDTLNALLSRAARYEHIQVDDVFLLFDELTALGARPDIASVETLHTVLEHAAHQPPEWRETRRRQLVELYQYLALEEIERLAPHRVDALLSAQIARLRGNLKQLNASLSPSVYRRYFAAIDLGETLIQEVHNFLWEYVGADHAAMDVPSLQLRIPFVASVMKRPLATADPAKVKATDFEDTDVCSVLLAAVERCVDGNFHDRRPVSERRMYLALLTMLTSSGVLYTADLMAQMMDVVKYSRDDRGRDRDAQRLLRYALRGSSAANDAAYRELWRAVAPPVDARVVGRYLASRDPWSPVHICYDRSFQFRAFPALQQITQSQCSSSSSSSSSSSTDAAAVAASTAAGAGSSSTAAAAAEPDEALEGVSAGPPPGTVAAKTAEALQQRWDDVRRLIDITGVLKPGAGLTSARTGSAAPTQEAAQQAMEVFTGAAAFLRGVATGCRYGELADALAIQAVGDGQQQHHHAPRATPLGGAAATAGAARSSSGNVNTELYAGGLDFDVWQRLMQCVQQLRQDMEQFMAQQYEAHGLQVEPEFECWEAMLVVLRCILDFCLVHTQQYGRTAGGGMAENLFLESAQLRAQLVEESRTRFNGRMRILWLQEV;> MQLSQNVARTTVPSYYHIRTNLPQRKPQNQWEGVYYYSGITKRQQHVVLLQRKREREMYLRQYNRQVASLRGQYAAHHEKPLASLPERLMFATKLASCGMHNEAATFVDAMHHGKELRAIDYVHLISSLRASDLGTCILHSEAACDPALTFKFLGDNAGAERATEAYRWYDMAMSALAHECGSLRPESTPAASQLTNALMRALMTCGYAHVKAIPDAVYDRMGARGISPTASTYDHVILALALTGNAAEAEDVFRFVRHRHAEHVTVHGYNALLLGNREARLFDRCDGLWQELVDRRWPRANPLTAELYLRSVVDHAYTPTSEGLQRFGSVHVVEKKKVPIVLTQMDELGIPRTHLSGPLRDEVEDALRKFSIYRNRFYEWGRAVKQFDFIEFRRRHGWMYDLHLMKNTTKMLPPIRDPSQPDSTMASAAMVELPAFFTERHPWERNALESLLSVTKERERMDDVRAGDIYYDDTKSIHERSSTWMNEVPETRYDQLYGINHPDVSKIGIRTHLEVEYTNRKEVMEKDAALVRKSIRRGRRLRHRVEVSRTHRNEGSLTAKESK;> MLAKYGDLTVVKDDLTLLEKTESYIAKWRLNRWEFRVPPLLYPAVREKVMLQQEILKALCLNRAEEHKHVLGDIQIVASITGISPESVREKNRAWLQEEASKLRWKGEVNKAKELRDAFLRLEVYGSRDHRLLERLCCIYGMGMQGTFDEAFSNIIVQDPSTGKLAVDEANPFAELQAYILSRYPQIDLIHDFLGLNVVSGYRPSLGRFLIHCLSKKNNISNPVSNGRVLLHVSTSKETLFDYGDSKNQVAHDDSIYGLPDFMYVRGNDIFLIIIAADNHWLRKRQVPHTKQLEGIARRCSFVLGIPFDKVRIRNLLLPPNYVDSSSLRRLTETVFDMSPASVKEAVPWISLYEKGLDAQDVDYCELEKTVNEEEWLTL;> MLRRTSRRLLGYTPINPDTSPMLMYSQCHWHYNLPQGMERPSSVNRSLPAPYQPHHSSVNKYRGVWISTEMHPAFLVGLAPQLKKLPHGRVVPQTPVAEVIDEFNKLSPLIDDAAARDGWLAKIFQHCAFQRSGAEAMALWDKHCAPRFMRDDSASAPPLPLVQAILFCCSKSDSAEWRPIFTKCLKDGWNYTPSFDTPQWSYLLKSLGRQGDEEGVRLVLEEMADVQADLDRVEARSLVYALNAVHDKAIYNYVKKYLFYLGERKVKFLRITYADLRGHGAEKLRVPLKENDSMFYHVCWHASIRQPRQFSPRQLYFDYAPSQLATSGHSPNAKVDGIVKDKIDKWKAEGLLPEDYVHEDRVYDRTAAFKSVARQEKWKKVPRIVKSKRFGYSGEP;> MSFRYTNHLVATLKHRLFLEAAHRQLVRQTFTGVCNGIEVTCTAYGSVVGIRMLDRAVWEPHYQVAADNKSEAAAATPTAPAAASPSRPSSSSSSSSTASGKTGIDLVKLSASIQAATWQAIQKVRAAKEETHSRSLRRNPQVLAEARLRDWYEQDANTLHPRPFDGLKNLEATEWMQAVRFGVPQPARYRRPNAAPKDLGEGGDGAHTDQKPRETITVLRDEDCDPANIPIGSVHPLFAPGLLQLEVDPNVATNGGSRVDEFFVLSEQRKEMRRDEEAFWERVELIRRSQLATIPKGGVKRGYADMADTVQDSIEEKVQLRFTQ;> MSPPALLRASGVLLDKSMFAAKRRVIVPIQPTPGYPAHFIKTSFTTDPLKEKQKARFSSGGDAMREVQDIPKRLEGQRSRAELTSRGDEDFAALIEFIQGASYDQLISGRRFRKVYEKLSENDDMFVWLCHTAMAVLNPGDMRSRLIHNHLKALAEAVASGEMTQRTAFRFFESAVRSPAYREIAARQLETGTATRLAGLAAAADVMREMGLTRRPMSSYFELYQRIVERSEAMTPWGFPPLFQFEERLALEPRLKFFSRVGQQQLERRRRGSIFSPHTILQGRRIFWIPPTWNRAGRFIGPHINLYPGLTPD;> MEVYRRIAERVRGALWAHHRRLMPERQFHRILAYVYNNKYEYQIRFDRMSVVGRAWAGRVEVMTTPGGFLKRVRVHPAVEDLSPAQQHKLVLAAYADACQQGRALMEQAELKVYKQFLQDLKPIILGIRDNPEFYTVPEDSVETIGGVLRRDQAPLDGGAAANAAGAVHRTIPMARAHQPVDEVRRRHAWEDQWLASKQGQRWAHSLRGKEYFTRHGPQYRPRGAPGAKTRTLPFELLAPYTPMDEGRLLRTNWVAYMDSKHVAESLWTRAKVADREKQLRQLQERGQAWHRPINEDAVQRW;> MLRTCRVLRFRMKLGSMYVDYKIVSRNHRRSIRVEDALVDPLLPTTVVPLHWLEQLRCPSTRLLTGYHTEEAVYAKPNYGDRVSRTPALLSLPDAAAKTADNGAHANAIRAGPVVLYITGQSIPVVLNPLFVQPDEWGLTQSNGEWDLRIGMDAIEQCSLYAELRPGGLLYSKLPHASLTEAMEPVQDTLKRYGMRCALAESPLVPRPWTRMRYMFIDELQRGQKMTEFVGYNPRNGTQWRFSQHTKYFRTGIWRETIRRNEMNDGLHAHSSWQKSPQQAVPEISFLAPYP;> MERAVDARRAIYELWSRTAAAEEHAQFSSDSTSTGEEAAAEAKAAEERSTAVAALLDKYKLDPATPREEDISRGLGDALDRLLLLCVPLSSRHGADLLVKLMQVSAQQGRQFSMRTIQHLFARTSSYAEALAVFYAMRRSNFAMSMEAYHAMLYSLQRLEEEGWAARFHEEFAASKGEAISEQALDFVLRGVDNQLMPENKPWLGRIMFAEVKDNKATQRQSMASFDAMGKLWVQRYKNGGTAPE;> MLSTSQAFLASLRYRRPYWMLFLKGADNWKIYTVIQQPDHQRTEMLYQAWLGGLDRPYVRPKCMAHQPVWLSKKRHLLQKARLEGPETSVEKYVLEWYKKFHSFQGTDRPTAEDLHTAFDLVERPLDLSYACQLLNQCRNHYYIRLSDDSFEIFLEACLRVDRRDCAIYALEHAEELGFWHVSDNCRRYLAGEQTWYKRSPVDLLYYPLEENAERNTAVTSGTAASAVAASDKVKGDEKVEGAPRTSATTSATAASAENEGEAEVTDDEIARLQAELEALEREIGSEGADGTDKD;> MRTQCSRALYGRSERGLYFPINHRIVDQRNTLGSGAEEADIQSRYRRQLRSSFVTRETRQTEPPAWSRSTRPTHFLSLPLPARCTLRVRVKEMHESMIFANQSIEPLLIPAAKLHVTLGVMTIGGEMVTAEAVSAAAAPDVLAAIQDCVGQACHDTCKEPLQLRFRGLGTFAHGRVLFAGCITEAHFTTLDTLVRRIRRDVGLGLGVDMKGNPHDSYVPHVTVAKIRPSQIGQFGRQLPISMWADHQHHDFGDVTFNRVDLCSMKGEGKDGYYHVVSSIAVQ;> MMFRGTSCALARSFRANLKYPSLVSYNKLPWEVVSHDSTKLHMHLAPNYEQLLTLAAVTDVPHLTLASHLIVPEAERLRVMPGVVYLLGGQAAHENPSSFTAYRIADPTSLQYYGRIHHNLAPIRRVDMCASADLRLLCLAMHFDGVLTNTSAGSTLDGVTTASQEGHFSLFYFFRPNRPANELTQPFEKFYRHRPSLASLDAFNAASPGKAESWTPVLQVPRRTAEKARLTPAEPYRPPQNYLMGLAERLGVRPGNAFGRRSLMWGTWF;> MATVAVEETGACLLCYTIHFVLKCIAVARVGDVLLTCAGTRSLWRTLSPLRHSLSPLFLSLSLSLFPALPGNCAYGSRVKTSAFSLTLPAERCRRVLEEGREAQGTTVAVNRTLAPSLLLPTANTNLCTPRGTLVEAMLRPTCALAAAEFKQKSRWSSVWPNMRYGSMYLNYSVGRQLPMKGVNWVTRDSNRLTNFAARYSSVIEDVDVKRNEEELNIQMSDVRWNDHRRIYWKCSFCGSSYRKNVSVRTKYHAGCNFCKGRYASEVLREQTPVVALREAQPELFKGLAENEKNDNIGSLSVTSKFRAEWKCQSCGQPYRATIRSRTGLTEPGQAPLHPRITEWSAHCPACAWRTNMTAIGRKAQEEGQYLGLETSLAELTGAAAGKRIPRRRKLVA;> MKAARLLFQSDRRTRHHMMIDGAINPREWFNWHPKEYQPWYFDRHKFIYEQGQYAAYNHLLCHQAYLKDIEHLTRYPEPRTFVIDCRMSPAKMHRWVPHSMWLPRDEVEYALQLTNDEFQEMYGFIKPAKDDDVILISHNGLASEQAGWEWRKQYYQHVYNYRGGTNELFGEDYQDFILKDRLDPWKGPYPQKSIFVDKWSKRKVLTRTGPFDRQYEMQDFALPDLELERPRHSEDGPRQNMPYGLQ;> MRRSLALCLHSTGACLLSAGKLSQYEQEAYESHRRFTESQTYPGPIRAATPGDTRFYMGSAETILQENERHYWRAVVDDPHVQHLVPLRVRFKTFIWVTSGWEQRVQVVQVMAQRDSTIAELMQQVRIENQSPYLCTSSFKLCIDGKDLDELKTLADYGIHEYSRIDAIEENDHLLHTEAERLKDWNVAEMPEDVLLRSPYKEMAMQPQPNLAPRYEAKPKGYYGKNDYSGMKQSS;> MHDANRFGGRTAYLREIGPIDHKKKGRLFKRDLPTLQFNVDVWCAQQTLRKQWKGRDWDVVEMPFEMAPKELQRVVPEKYTDVPIMTDPARHDYMNIRRKVFDREDMQDALFASGGAGQSPYPAIQRVDKAAMTLDKYL;> MRRTRLVCTATPEKFSILGTTHPKPKRNGMGRNNKMRSKPSDNVAWYDKGPVEWLPRPVRLTYDQLDQLRDWMMRETIAGRTEEFNKIRHLHREWSQHPLMPVLGDVEPKFPLNLYKQNHRAKRRFLVRWHKANSPTYWMWMPRGPAVATPLHRSSPSQFPEHWKSLARTSSSSSSSGSSSAAP;> MNRSFVSSADLRGLTAAFCGSLTCQKRFWAKPKKRPKVGPGFHEKAQKWRDEYLLDRHRVLADSLRAYVDFSSTKRVEPWDTRFAPFDRVEKDGVYILTRYLMDDKLQLCNYHHRPVKRMLCNVGLMGPQVTTTARWKPYRFATNPANTTRAERTFTKDKTVFTGYHHD;> MLRQTAARLNTYLTRSVATPPISVIRTGPKWWAEPERMVKHKVMYFTMGIDQLPLRRTAVIQKDLKRFHMCKPPPRVGDATGYKRSRGAQLTTWYRRIQYQEYHLQHLFVRHMWGLLRMYPGNTTKIQGKADDGYVGYDSVHFHRYNRSPLPFPAREIYERRK;> MVFYSLVLVMKPRPRKYTSQALREIAVNIYNHGGLIRKLSNEGILRPYSRFRDADNTAITYARYVTLQLDMGEEQMNKVEKIIREHADVNITLRLNNLERPTGVKHNQQSAAAYFPLDTFTRLEEEINWPPQVSGDVYEQLDMNWKEFSRTRWSNYLRN;> LRRSNRWCMKYANLELTTRGEFPHGMKEPGFVKKLDKNIPWYFSTYRSMYHWPVAGDGWSDLNEAEKHHDLHMYYTLAWWKLGEGIFDADDEDR;> TKKGATKILFIYKLSKLNVYNNESYKIKLLFNHLYCIDNYNSIYFNLNGILIWLNVLHINIILIKYAFLILLNNLEYLIIFKYNIISIK;> MLLRRATRLARVYGGGATTAFVPGSSSSSSSSSSTASVGADYLRGRSIGAKALLGRRARQGSLFAVANDVTVSEKRVRQQLNALLADERDPLAEARRQSSAAEGFASSARPFPQRPLVNLPGVERVRDLPADPITRLFFQHQGDHALYYGTYDEPSRLDEDRVQLEKREPKDWTFNVFTPVYDFCHRLREASEQRKRFVIVPSTIETRGCAKVLLDHGLVAGFRDFRNDRAFAVELKYFQNEPTINIIEPCSYDGKTEFEWSPKMMRRLMNAHGIHNRLIIYICRTADNRIIDHIQAVKECIGGRGLMMAH;> MYPGEYVPAGHNTLSSLRDELRSDLTAQSLKEAWMRVSGGMYFKSIDDYYASVDGLDQEQLGEIVSALLPDLRKYEAQALVTKVLESLSKPADSPSRQLSRTITADAVGLDNAPGHYTNFLEWMGRMTETKAFKTEHALFEFSRRKFNREDVRVMFENYNLMSKATLEADSTDSYSHFYTVLHDFSRKVAGEDTRHQIGVRIDPAEVDPETGIAVGHGRADGQKYMFTALIRENRDHNGSVTLLGKPLSVAFDDKSWLMEMVLMPFDEAKLDFRDFDVNLISEGKAMPSFANEIAAFACRMAVANAITKLLPLARIPLKKAGLLSVDRRREPGQFPGFVDGKKNKRKFAKR;> MRRCTVARYYWSRYRIPSQMPKFDGPAPVAAPQNMNSTKTNEFIDPIDDKFPVTIRGNLVRPDVPEDQYVDSWYVCTSMTHHLGDFRPWSASAPANAYRFRPYNEFDSKGREYVEHLRKYSRYTPQASRGKGANGFPFREAFLTKMNTAETAAVNPTRETVMTRAVAERLHHARVLSPLEVQRDVGRLEEPLPCAGKIPAERSTFPFRWNTEDWYEYEVAKARNKRFVFENTNDNGVCASEVTYRIVLEGFWDHHVMKLADDVVMFLKDVGRQVVDEKLKSVRASLESLSSGGAVDPELVAAFNASLKGPFGGADRYDADEVAHFLRSELERLEEQCVGLINRANVPIPGTSNIYDANVSWPHVEKMEPWTRMAEFWTSSSDTSFTELEMSTAHYEFRKYFRVVVVKMPFQSTEFEQRMYGIRHWLHRQTSCEFHTTYRRNVVHDSAVFPTEHDPETKPSHEHHRLFSFALDWQSAPVDYLSVELAREGDSWSSLAKRLGCSESELKAANGAMEEVVAGVAVSVPGSATRRLTSFSTTPSVLPLQQGDGKPAITSWRRAAEVLGCSVEELQQANGAAALTYMAAAESGDGAFDPAIKELVVPHTATAASPESSFAAFEPVFEGDTWTSIAARLGCSEADLRACNDVDGSVADVSSCASVSVPASATRPRRIIHPQLRPQAATDALLARTLGEQAVSAMGDIPSLPANAHKFPHEYHTPTSRFPTTPQQSPASDNWIAYTAKYLDKQLALQDEPATVYNVNKLWPMQQVPGKVDQTPFEEDQTWLMHPIPVHQMQQHHPEKDLQDLPFVNHEQFPRSLEWTAP;> MLKSSIVLLRRGKPRPRAGMFPEKYRRVPTLLKPQQGGQQYFNEFLIRSANDALEAQQQGYGSAFRVGGSGAARILADGNATAADGIHDGEISSVHPRLPQADIDGVLQRSRAETIQAELKQLVAQDGFISQRGFNERLWYEQEHHRLRTHGDGVEASPSEVAATAAASSSTAEAVSATGEGRAVPERILGDDYFQSKFGYSLLKGRSPDASAVADNVKAYAQLDLWGEMPMYSRDFVFLYLVSRRRNTYAVAYDYDGKRLLPTYTAGNRGLKGGDRGFRGDGSTDNGHQVTSMYLNDLLPKIREARAASGRPLGRGEKIDLVVRVMGFYNGRQGAVRAVQDRSADFRVRYLEDVTPFPLNGPKMPRGVFR;> MQCTSRLLGGYMMYHRKSMSTMRYSKWKGARGGLSHFYNRTAMLEKVPVNMPVSIVDRRMMAYVHRSRLRHFQLFRSYQQKSNSTECKLREGEFLRRRWHRQLQKSFIAFMQFKTMKVLEEQAKLVSQYGQASVNAALGDPQAAAGDVAHERKYAALHRRVQTLPRIQLVPKHVATMKQIHNDRFNYRWRVN;> MLSCKGVLLMRHIGQDVPRRHTHFVLESRLMYEKSFRDEWLRSLCQGLANVDEPLAKSLSGLPQQMLQRKVTCFSYNQFGLFKVPYYRLANVDRYYAVQGALGTREWVPYANVSSWTMNKMVRSGNILVHRVHYKGWGTDNALNQGGWEHRWNKVMQRNALQYNRI;> MLSYTSTLLRVFNRKNKAPQRMSNFTKVTNLNKAEKVKIETVDGDVVKGRGRVHRRSHSGLKDAIEEMEHPAIWLWYPWRKNPEPPTPFMPSQRALKNIHGAIFANLSPIQKKKQEQMLYGVNIPETRVMRFEQQHPLLSTALTQLDGQPKGFPFWYKKYPTRRHAYEQRFSVPTEMLEGYNDSIKKAFSMSMMTIQEKQFAQEAMYMERYAEHDFDTTSPAVLAVKRALKVRVLRNHLLTNPHNNIVKTILANTERKLNHTLRRLRKVDFKRYWEIIRDHDVQDVLQPPNLVTYRQGSYWRYDWNAGLAISTQLADVLDPRGLNGCVETGRSRSEVARDLGLSYTRPLQENEKKQLSEQAVYYERLAKFKMEQPEAARAQERERFVRKFSGMFLKLDMKSGVPDFPSTYRKLLGTQVARWSSKRHGPM;> MFSTNTVLWARALVDRKSPQLWGAPGAPIIRMRGHHVTWKFQSYDMFVEHTHRRRNSDIRLLHYLGKHCPHPQKSLWSPDTPVTQDRHLFMLTTIDVDAFKYWFGVKRCRLSVGPWNILAKSGLLPPSYKQNSKIMPKPIFDKEQLMRYYLANRKDQRQMEREDYLNYKNSMVKSPEERAAERPVAPFL;> MFRQSLLRLPWWNFQTEHRQRCVMMYGGARTKNTHNANHRVYVRKFKRNAFPNRTRHHWAVSMTGVQGQRPRRMPWPYDLTSMIFNQPRQGSDKIGYVVGTSMLKTAVVAANHMVYYPKFNQRVSRTSRFFAHDEDLACVEGDLVHIKQSRKISKYKHYYVFSILEPNIEGRERLKLGLKAVPPPLFGYPVSRRVVKLNLTNTEGTKEKLAAAIQEHVQDAYRFAGPTPDQPRAKLTDSASFDEANKMIAPNSSVTAELPPGAEPAFLGDGQPVAEEFSEVEEDSRHKKGDDYWMNLQPSDKYDFKNLKKSP;> MITNPGPLRVAYSPDYLDWLYRAYRSKLKYTDERKKAEEVFNGLLLTNQTDEQGPAAGAALPGAPPPGQTLRPRHSVRRQAGEARRAAAQAKLDTLAKQQGMLDLFERQPQFPAIHIDKAARFHVVELFKEMVLDRAWKPEEVWDKALLYRAILTERQASYPASYRYILDTAQRVNLAPRESGSSDTGSSSSSADARSSNESAGGIVSESTLVIPREDNYMYFVYLVRRYYIDNAVEGHVVLRCHRQPNASELLFSHPPPKDEHEVLRSLYRPGTATATQGKDASAKAQDGAATAPQQRPSGAATIARPRPPSSYPPIEALWRCEENEALLRVLVFGELNLLVSENPFVRFPKAQAYLTRPSASTPVPGAAGGSVEGADGYGGPQQQRRGGGHRGIGSDGGISLSSVIAEKRGHLLAPLSRNVAMMIDSRANDVRRLQQRYEREDTASFQKMLRGSAQVEENPGLYSAYSDWSYFNPRAVRAEERDALSRQTVAALKTYDEASRDIYRVGFEEAEARSAVRPVEGVNNAPSYVPTLPHFVALVKKDPHVSFLSHVALPEVYNTASHAAAGVSAKHQLEKLVVQLARALYRTALEFHKEQLRRVNRQKVQVAASLLDRFVTERWRVHCVAHPSSEGVRDMARRFRAYVPFEGRILDESGFPTDARVEDYERWMAAPSV;> MNRIPAATRNAPMYATAMSQFAVCRQPWNEYISLLTKDDAQPFHTTPQEKPAYRGRKRGREGWLFGQQVQLHYHRFPDEQLFTNLTRWRMGDTVGDVAIQQFRNAQPFDIEDKDPQGFQRPAPEVYMKLNYKNPATISRFLTRTGHMYPQDIMPLNPEAVVKLRVAKAQAIRIGLYPRFGNPFWFRSQSFRPKAYQENYDPTTYSTKHTMEHFAYNWVQTDRIRQYFKGLEELHQSRRATASSGGGGVTSEHKQQSQLYALDNMSIEMHRNAPSYRADVERSIKKPTVPGLMSTKGMKKKFHNLYSSTSTKRMGFSNPTLGIKKV;> MLRRCASAVAPAAHIPSPAAAVSGVQKRFLKIAKSTFGFYLARRGQRKFPFHRRPHIKNTQAMNLNAPYFWSYMTAKSQSFFLPEENYITGDWTGKFFVSKRQVYTLQHATSGGKVRVKSFPSVFELNSPSRWNVGKEMNTLTKPRMDLIDDQMLTKKQRLDYVKAGLLPK;> MLRRSALARRYPFTKRGPRERKSWKHHVLTEPPKPVEWRDPKVWTKDLSQMKSFDAPQWDLWLNRSRSQDMDEALQPFMDMPQSLKDRRYDIPWWANPFGAWYLQNVLSVELMKLPGRTNAEKIAIYRGRKRPATWDKSKEGLMDDEVLLKQIVKERWRTLEFGDRDAGYPCTFSDYIQFLNEWFKSLDEEGLQRLREHFDRKIRPLLAVMTHVDLMWLEALTQNSVQNKEQLERRIGFQTSLGTPEFFDMSKRLRYEINEDYKVRDELGPELFALWSKAPERWPPERLAKMYGLDFTLVRKILVWHHFKACYDACVEPDWTLPKRLFALEWIRDVRARKQGLFYGKLRFAEQKITFYSDKFLFRDLVNRREASYANVWEMDDPYRFLQTEQDYEDYWGDNYDVYRRMFPEMIGKSGEPVQQYSQMPVWAGPHRDHANKSEHNWMFAEIGVNVGHEPLKKLELDPTNEKRRRFVIRQPDGSLRSAKMSEMRAWYWKEEWADFRFWAPHMEWGVENTPSMEQYQEHVPDTPDADYRKQRRIQSRPVKWFYESHYSRSGSFAGFQPLRFMQRRTQREVRWPDVINAAVQIEKSKPSSYVFKAIPEI;> MRRSSSCLYKIPKNTGVAPRFDTWNEKYEPWEHLKRMGRLAGTGFYIPPEWYNHFRMFPPINHNFQQEKTLNPHNVSEPTQDDTDYLSVERIALRDELARKSRLLASEGMRYYNVFWIRKPLDRMERHYYELERKGVAHSVAIKRVLQMFYDELTVKKRVAAIQAEEAKLSGKYISMREATVLMGVLTQLQKEQLTPHQVTLLAKEQREKAQAGEAFAATVERSTETVADAAKDAAEGDEVMSADSLAELLSTEADLDDSSPSISYKVTIHETEHDSVKQLQELALDHTGKSDWYTGASPVLHMEEAMPAKRTPASKKTES;> MHSSGVARRQMRPYYNLPSKSEHGRRMTGFLTPYRHWMWKQNELWRNVHEAQFEHLRKLYKRQWLESFRVNADEYIYKYNITKSAQLAQWEHEMQGQERKRRESQQLAQGRQALKKKHLDLLREFHERQFFYWYERASERLQYMTHINYVPQASIQEHIDRELDKYTVGSKAPYPLNFVGQMPMLEDKDGNIAQVPANLMTNHATENPDGGVTMYEAPEGTAVAEEKLLQMIASAQEEELRIRPEDSDALSESMEDMDRSESARIDSRKVARTMEETDEEREVNRRAYIDRGKTGSKTIFRRPRLDSDGATPPSAGGTTPMKRRKSKMDRMHALQEQQDAVAAKATAKALKDEDSVAKATKRGEVAENRGRLRDRMIMPSLETLQQSPEMMAQNKPGGRVRTHHLMEKVYGIGKFKKGGGGDEDA;> MWEGAIPLKHERVLNGGVATRVVKKTYSHPPEIHPTNLSFNDIDSMYCLGNDELIKYFPEGVGGKMMQLMPPGHPRGFLYRKQSHLLNCFIDKLPFWQSKEKALRSLTNGRPGFIMDGPTGCGKSALLCQAVHYARSRDIITLYIANAKAWTHGEWCWPSTILPGFFDAPDAAREFLRTVAEANGSLLQAWELRVTPQDLPLEQGEKQPRSLYDLCEWGHRAVAPASIDRQSVCIKFFFDEIRAEKTKPIIIAVDGWNLFSHETHFRYPHPDFLRTLTTLNDGLTDVDLYPQELPRIPASRLSFVRGLNKLILSKQDPNKFFITCTTRDFKPFDGVSGFADVENDRFKNSLDEYAPYDPEKDSFFHPMQVENFTEYEYRAFLRFAINSGELAGLGWGPMWHYSSDFERKLYKIDFMSDRNPQRVVDHYHQELVWRYEYKRTRQKQYLLARRKMWQGAEVSNPLRNGK;> MLRSSLRYGVHKVGYTHPHHLPVPCAQRWDLRLARARIFQEYIEEKAPGAWQLEDERHMSPEFNTFTGYPMRNLRPGYGQNLPEFIMKKRLPNNTHYELFARRDIPNEDNAMYGKLLYDMTIHGTSLPSIYRMHKDINKAQRNDRKLSGNRFKVLNSSGAKSPPSGFEAIPDAVEEEDD;> MRGRTLTLLARDALNAGSSMTLGSKGMRPSPEAHRRRMPWTAAKEYVPGVVLNSKEKLVLDGTQLVELDHIDRASQVDPLEVLKAAVATRAYNTSTGFNIFQLASQTRFHGRGQKFFREEWRQGTYEKYVTLAAIDFDREGSKGTAYGYITFHGESTTRPVEINYADTPGWQMEYDEAAAVPFDAAVPPPPSIGTEVPVDPSTYRLKAYPFYDAPNPPAFVERLLKDRGVLPDLPMDASAPAENAAAASADGALVDGSHHYESKGSV;> MLRFPKQVRGGHGTCRVALCSSCRGVALTPQRMQLQHRDRIIGSHGAGLVNHQSMATMEIRSNFTRVQNAAPAADLFRTKVHEGLGTSDKDPYLRTLPNQESRPPESSVLRVAAATAPSLEERQCLHQKWGTLQYWLGDQYPRLPLFLEELLVSDALPVSPAAEAMVQTFAAEVIPAMAKQGGPGAEEKLEALWKQAVQAYGKLTTSHVFDKVAFERELAALRARYQADMSALSPCEDSALALEVLRRKAIAKRNAFLREGLLPMVRNSPYVGYGDGVWRVFFDSVAAHKRDLFSSSNSPVSATLGFAWEGLMMEDAVRTPAMTAPVALYLLLVSISASHNRAPAELKTASAHLDEGIVSTEQRVVPSAFATVSPIVKRRFAADALKGLLGEVKGCGRLAKALRSARLYDWSRDAALCEAMLDDRQLLRADVENMVDRFDSTAEVKSLLQSLMSGTDSAIKAHVSHVFQLPGMASKSHQLVDWDATMSAVDWPHCWREHARELLSDPATLEAVYRLLKNATGAKHATKRLFSDEYAAEVEAALQRRKERAEARKARAEQLVRNLTSYEQVEGTLAVLRKVGVSLRELEGAELATAEQRTVRRPQVDNGVLDLLLEAIRQRHPSWAKSGVLPAVASAAAKSPVWYLECMTRIYIRLSYVPQAAAALMAQRTRRRLGPVGTEPTQFNVPTEMGMVEQYDNLQYKRYDWQGWYQRMVDVHNRNVSIKCRLDDLKRLDAYGNPFVEMQTERRLRILADHRVGMGVLKLDSDKYEDQHDNITYGSTKLSELLADARKAQLGKEYWPSVEVKVRRPSGQSKAYYSVLDDARIESKSKELYAKYREAKKRSLFVTPMDLWLDVKGMQVRKAAETADAQGYTVDSLQYAMEDDSSDKG;> MKSSDIFHACKYTPILLKSRTNDSGVNQYGLRPVNSYDYLNPTNLVNFGRGTAFDNLGVRRSERGQIDSAPSLGGSPVFTQAKLLGLSGDDQLRLCEAETTQLRMCMAKGGSACERESLLLDACLSKVGHLRRAISQAGSEFNDWFIQNVSDNHTKPFQHRPHDWRHYYAQEKLVREKQQNGHAYGRRPKEFSFGARYVKTEGYGKRPRLPYNK;> MRYTARFLDQTTGPHKAYKYTYMPDPRKLAPIETSMRSEVLPVVIRPPTSYVPNHEVFLEKADVHRLAPTSDFKATFKDWNDLMTCSKRELRTRGVPLLTRRAIRAAVLAFQNGNPPERFDTKEEWLYYKQFKTKDYSYRVVPELPEKYRPHQNGIDQAPVPNYGEINQMPQWAVEEEKRLTGKISAASK;> MRLSLLRRFCEYVPKGAPTQVSLSVETPYGVTRAFRMTEMAAAAADAERDAKGFFYLPRMDYDVGQGVAPLMSRKQFDVQYNVFHKAAVDRLNAHTLGSELEGHNLNVVIRNSSFDASHAVIHAAASEHFNYCFWYRSLRPWGTAVPARLKEELQLQYSQNGTLDAVKEVQRLFTVAALSQQSAGGWVYLVWTGKAFDVIPFDHGTCPIGSDLIPLLALNTHESARCYDYPLAAEDEEGDEVERFVRNFFKTCNWRLVEHYFLQCGRA;> MRPEAAAAELRRLLPLLSFAGRRTGAATHSVASLIVSTAYSATAARSVTNHSRDCPVLSKKLPLPLIGKESSFAARPCLNCVRERVHYVSSLSFCDYFEKKCAEAQHYRNGASSNGVVGTAALPKLLLEAIERSYGSVAAFKDSVMLHSTGAMSPGRLWIVYTPPISGSEHGAVRLLNLPACKVPLVHGLWPLAVINMTEKRLCEQIACRSGKGGDAVDADDAPAWRHAARTRKTLGALATTEEGNDRAGNVAQVKLSSIQSAIAEEALCAMNWKFVETQLTSALAYYSSKERTQTQREHRKEKEHVAAVRAMSQLKNSGAVIHATDSVTITSSNSFVASSASEPNLSAAAAVTSSSAKAENSALGEANTQTAAVAAPSAEATAANTASNSAQPADNTATGAAAAEPRAVQQADGTWEYHYNNGSVTKALPDGTKVFQTESLTTTVFVNGDTLFEYPNNTSILDRADGVRVITYADGTKKEERLK;> LRRRVSATPSLAVSPAGPSSLSLTPSPADSQQRRSLKTLDVREYRPLGTPIEFRFYQRYANHPNRQSGVQFLTHYNTHQRFRVNKDFIDYMHWGKEQGQARLPHRHQRVAFDFDDSLQPTRAEGAVGAWFAGQDPTMRSHPDISASFDPNKKLFSHPEHWNKMFSKRRPGEGDIKLNVIPSNSLLGPMVTQTDTQDMAYFKTETCGPTHGRVPGINAPFKGEMDRKMMQAMSRPLNRSCTLTGNNGRFSNTIFINDPKRHQTLSATLAKELNREVDRATNGLYSKLTVLTSAQSGLTDFFCGGTDLQCIGFDLTMAQLLRKEADALTKSAASGSKKVEAKVHELLRDAERYEERADSVLRENAAVIWRAYTSPRALMTLVNGKCRGTGCGLALAAKYAGLQDASEFIVDGPNVGLTPYSGMTRLLARPETSLKYPGLAEFVMLTGASLFAGDALRLGWSDLFTSLPDMPYHIKDWFDSTEHMHNDAVAWQLGHLLEKCFQMKDRWHTSAMERCAMTPIRARWVEDAFADQSSIEEILKTLSAMEKLPLTDRHNTYDPSYATPYTLASVAEGVEKLGASRLRYTLSPWDATPPEEAVEVRQAAEIFTSYVLERRGKVNIVAHRDRHKVQAWQKQREREYVAYSNMKNAPHRRHVYVRLEGCEGTLVDFDFTIDPAGDAAAAAAEKGAGVDDRNELVHTASVERLKRAVLQAMGMPADRDVDLCWYLPTLDTCPIRNDEELVDVLHSDPGFEDPSAQLRYPPIYFLVKRNTLHLSEWAYAVKHQLLLQSPYALKATLQLLQEVRGDGSAKAVRSLADTLATEYRYAARLLKRPDFYQVGQHVDKSPEEWDVVKEERMRYVHKAHLPTRPLPDYEVVFERNVQLDGHTFQLRPRWSPRTVQEVTAESLAPLATPLDFEKDGAVEFNVVVHASKADRLAGMIEDAGGFEVVAHLGEVDKEGNAKVPPLHGDAHVPTNVNFYEMARHPWEDTPSSTRRDGFTAGSKEYFEQQYKKAEKAVYDEAGRGQRNYWPSKAAVDGVTGEESNALLEERFFAKLRDAERGVESWARQLRKKAVEGKLDNKPEIATQQEKIYDDDYYRWFIQPGHNPNPSGLLRGRKVADSGSSSVDKDLEVFLNQLLSGAAERGADGTTGDEGEALSLPEEDTDEAADST>LAGLDTAIILIAFIITAAVLAYVAVNMGLFVTQKAKTTINKGEETASTAL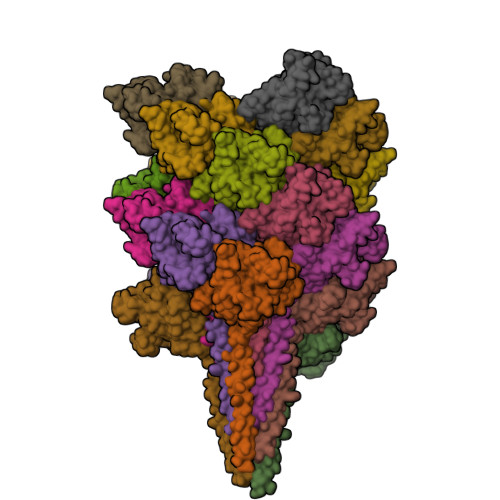SLSGNVLYAVNYPTNTKSYWMYFTVSPSSGVSSVDLSPSTTAISFTAASRGVSLSNIYQFSLLSVLPSQVNNKVQVKLGTSIINLTLAFSSNSAGQTYVYYSDPNYALLALNYTLGQEVKGGQLTSSPLYIISNTSIVASKPWLKNDNVFTFNISVNGTEVEYYAYVNKTFAFTYPVSGFPLAGSDIAPAGSVIGVMILFGPGEATNVFQYETVTIQITPNIGSPLTISQYIYQPDGKVTVIG[20x]>MMNYRKADMKDISLLVSIR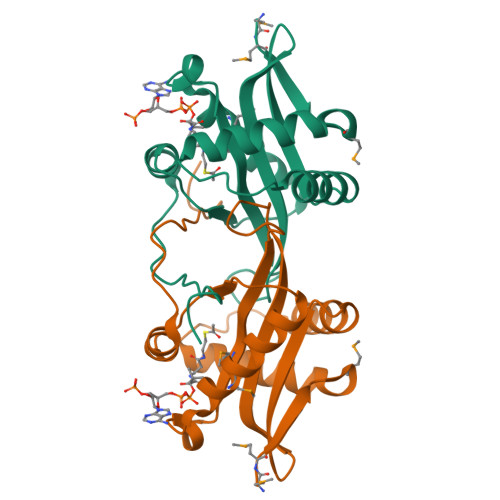KRQLIDEGIEPNIDIDKELTRYFNNKLANNLLVEWIAEENNQIIATAAIAFIDFPPTYTNKTGRKGYITNMYTEPTSRGNGIATGMLDRLVNEAKERNIHKICLVASKLGRPVYKKYGFQDTDEWLELNLLEHHHHHH[2x]>MKGLVELGEKAPDFTLPNQDFEPVNLYEVLKRGRPAVLIFFPAAFSPVCTKELCTFRDKMAQLEKANAEVLAISVDSPWCLKKFKDENRLAFNLLSDYNREVIKLYNVYHEDLKGLKM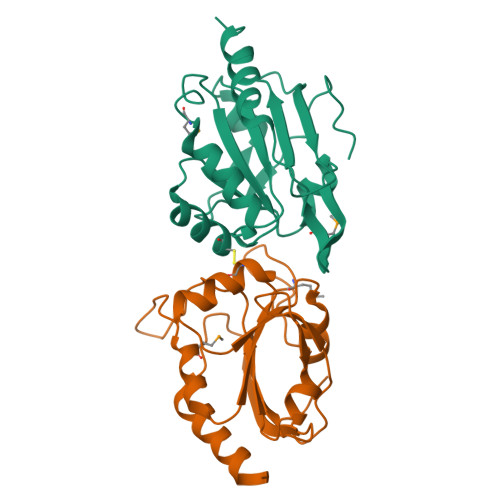VAKRAVFIVKPDGTVAYKWVTDNPLNEPDYDEVVREANKIAGELVA[8x]> YEVKFVEAYASLFKSRLSKLKRILRENPEISNVVDIGKLNYVSGDEEVTIIGLVNSKRETNRGLIFEVEDKTGIVKVFLPKDSEDYREAFKVLPDAVVAFKGFYSKKGIFFANKFYLPDVPLYRKQKPPLEEKVYAILISDIHVGSREFCEKAFLKFLEWLNGHVESKEEEEIVSRVKYLIIAGDVVDGIGIYPGQYSDLVIPDIFDQYEALANLLANVPEHITMFIGPGNADAARPAIPQPEFYKEYAKP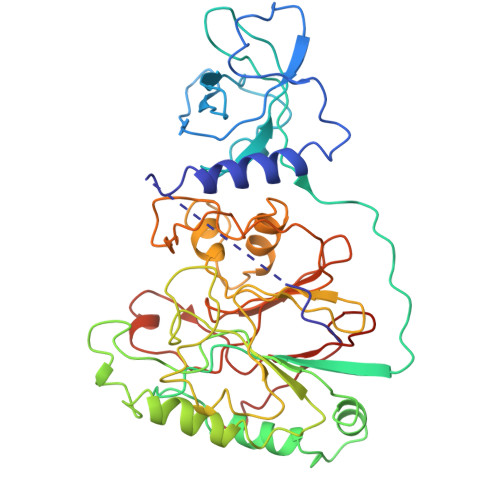IYKLKNAIIISNPAVIRLHGRDFLIAHGRGIEDVVSFVPGLTHHKPGLPMVELLKMRHLAPTFGGKVPIAPDPEDLLVIEEVPDLVQMGHVHVYDAVVYRGVQLVNSATWQAQTEFQKMVNIVPTPAKVPVVDVESARVVKVLDFSGWC> MNRRVLVTGATGLLGRAVHKEFQQNNWHAVGCGFRRARPKFEQVNLLDSNAVHHIIHDFQPHVIVHCAAERRPDVVENQPDAASQLNVDASGNLAKEAAAVGAFLIYISSDYVFDGTNPPYREEDIPAPLNLYGKTKLDGEKAVLENNLGAAVLRIPILYGEVEKLEESAVTVMFDKVQFSNKSANMDHWQQRFPTHVKDVATVCRQLAEKRMLDPSIKGTFHWSGNEQMTKYEMACAIADAFNLPSSHLRPITDSPVLGAQRPRNAQLDCSKLETLGIGQRTPFRIGIKESLWPFLIDKRWRQTVFHAENLYFQ

MAT (methionine adenosyltransferase, also known as S-adenosylmethionine synthetase; EC 2.5.1.6) is the only known enzyme that synthesizes SAM (S-adenosylmethionine), the principle methyl group donor and precursor for polyamine and glutathione synthesis. The function of MAT2A is further dependent upon an interaction with the auxiliary subunit MAT2B, encoded by the MAT2B gene. MAT2B is present only in mammals and bears no sequence homology with the catalytic MAT1A/2A subunits, but instead harbours signature motifs of the SDR (short-chain dehydrogenase/reductase) superfamily. MAT2B was proposed to modulate the catalytic activity of MAT2A by lowering its Km value for its substrate Met and the Ki value for its product SAM.

Limited proteolysis is a valuable tool to remove disordered or flexible regions in purified proteins, and can assist in crystal lattice packing. A small-scale treatment of purified hMAT2B with limited amount of trypsin, chymotrypsin or subtilisin generated stable truncated products (asterisk). The purified truncated polypeptides, found to have molecular masses of ~28 kDa (subtilisin-treated hMAT2B) and ~32 kDa (trypsin-treated hMAT2B) by MS, were subjected to crystallization trials. The subtilisin-treated protein (hMAT2Bsubt) yielded diffraction-quality crystals allowing its structure determination at 2.2 Å resolution in the unliganded form. The hMAT2Bresv and hMAT2Bsubt structures are highly similar to each other (RMSD <0.35 Å), and can be structurally divided into two domains constructed from discontinuous stretches of the polypeptide. Minor structural variations between the two structures are found in a loop region of the second domain (residues 282–289, loop C), forming an extended coil in the hMAT2Bresv structure and a two-turn helix in the MAT2Bsubt structure. The importance of loop L1 to NADP binding is also evidenced from the MAT2Bsubt structure, in which the segment Phe60–Ala77 was not present in the structure (probably owing to subtilisin proteolysis) and no electron density for the NADP cofactor was observed despite being included in the crystallization buffer. The hMAT2Bresv structure did reveal a head-to-tail dimeric packing for the two NCS-related protomers within the asymmetric unit, but it probably represents a crystallization artefact for the following reasons: (i) the C-terminus involved at the interface is partly derived from the vector-encoded sequence (AENL; residues 335–338), (ii) no equivalent dimerization is observed in the hMAT2Bsubt crystal lattice, and (iii) size-exclusion chromatography of full-length hMAT2B does not reveal a dimeric species in solution.3-[6-(2-azanylhydrazinyl)-1,3-bis(oxidanylidene)benzo[de]isoquinolin-2-yl]-N-[2-(2-hexoxyethoxy)ethyl]propanamide | C25 H35 N5 O5 | 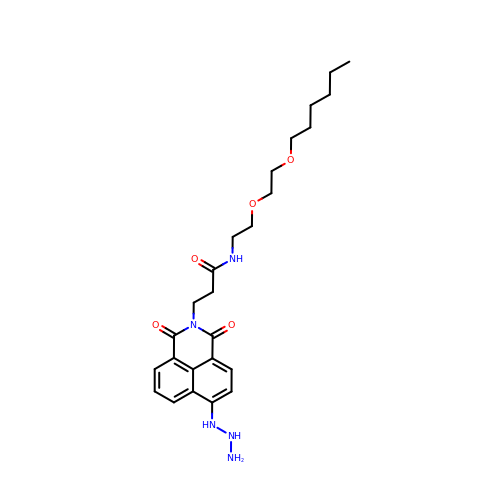SKQKTNKUYTUXKA-UHFFFAOYSA-N> SFIKPIYQDINSILIGQKVKRPKSGTLSGHAAGEPFEKLVYKFLKENLSDLTFKQYEYLNDLFMKNPAIIGHEARYKLFNSPTLLFLLSRGKAATENWSI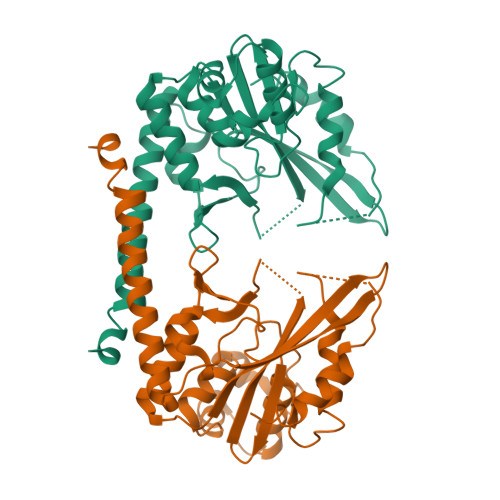ENLFEEKQNDTADILLVKNQFYELLDVKTRNISKSAQSPNIISAYKLAQTCAKMIDNKEFDLFDINYLEVDWELNGEDLVCVSTSFAELFKSEPSELYINWAAAMQIQFHVRDLDQGFNGTREEWAKSYLKHFVTQAEQRAISMIDKFVKPFKKYIL>EPEPWFFKNLSRKDAERQLLAPGNTHGSFLIRESESTAGSFCLSVRDFDQNQGEVVKHYKIRNLDNGGFYISPRITFPGLHELVRHYTNASDGLC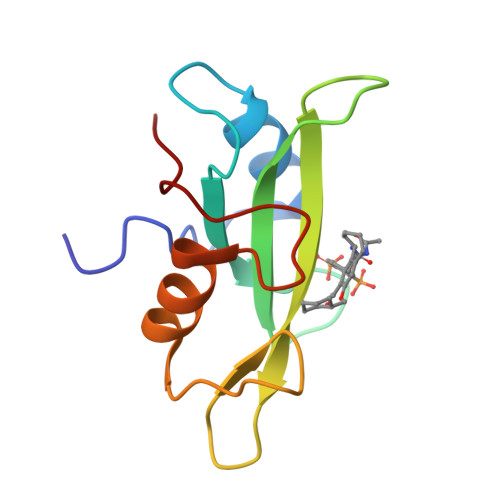TRLSRPCQT[2x]2-chloro-N,N-dimethyl-5-[({2-[3-(prop-1-en-2-yl)phenyl]propan-2-yl}carbamoyl)amino]benzamide 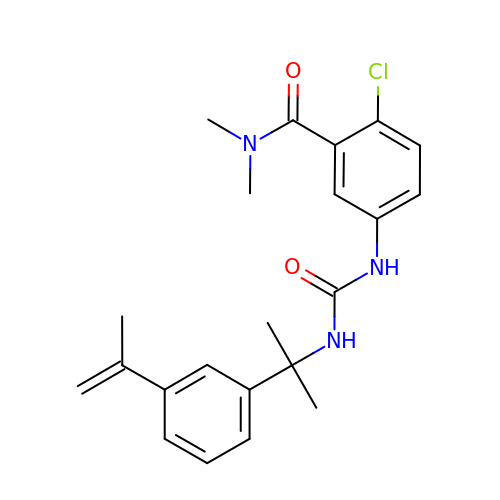| C22 H26 Cl N3 O2 | ORLSJKGKUHETDK-UHFFFAOYSA-N> SNAMTHSVQLKILDKRLGSEFPLPAYATTGSAGLDLRACLDEPLKIEPDETCLISTGLAIYLGHSNV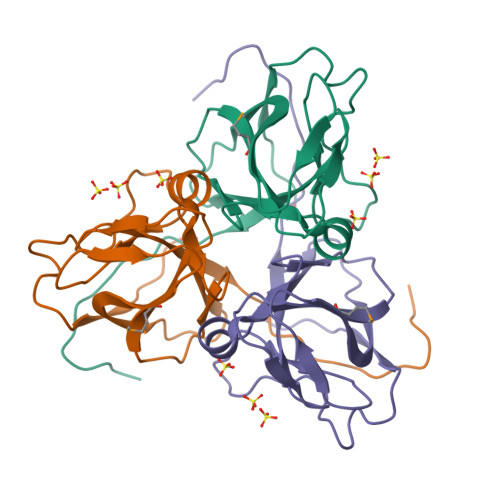AATILPRSGLGHKHGIVLGNLVGLIDSDYQGPLMVSCWNRGKEPYTINPGDRIAQLVVLPILKAQFAVVEEFELTERGAGGFGSSGQN>TREARISRAKRAFVSTPSVRKILSYMDRCRDLSDLESEPTCMMVYGASGVGKTTVIKKYLNQAAAAAAAGGDIIPVLHIELPDNAKPVDAARELLVEMGDPLALYETDLARLTKRLTELIPAVGVKLIIIDEFQHLVEERSNRVLTQVGNWLKMILNKTKCPIVIFGMPYSKVVLQANSQLHGRFSIQVELRPFSYQGGRGVFKTFLEYLDKALPFEKQAGLANESLQKKLYAFSQGNMRSLRNLIYQASIEAIDNQ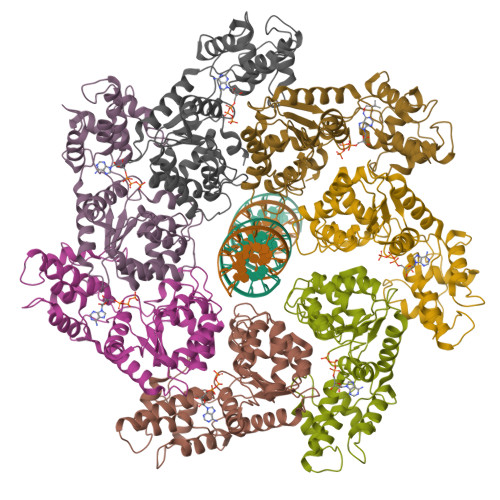HETITEEDFVFASKLTSGDKPNSWKNPFEEGVEVTEDMLRPPPKDIGWEDYLRH[7x]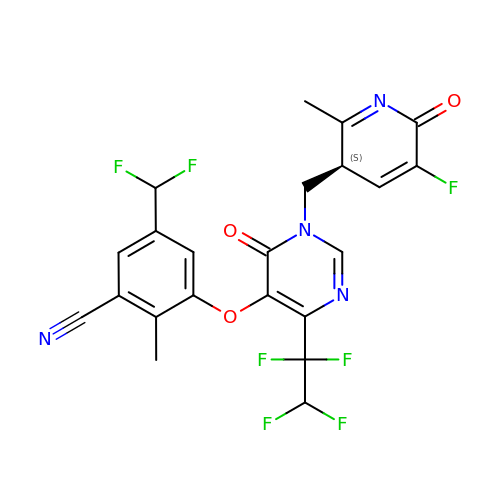5-(difluoromethyl)-3-{[1-{[(3S)-5-fluoro-2-methyl-6-oxo-3,6-dihydropyridin-3-yl]methyl}-6-oxo-4-(1,1,2,2-tetrafluoroethyl)-1,6-dihydropyrimidin-5-yl]oxy}-2-methylbenzonitrile | C22 H15 F7 N4 O3 | YVSVCEXZEPOJHL-ZDUSSCGKSA-N>MMRLRGSGMLRDLLLRSPAGVSATLRRAQPLVTLCRRPRGGGRPAAGPAAAARLHPWWGGGGWPAEPLARGLSSSPSEILQELGKGSTHPQPGVSPPAAPAAPGPKDGPGETDAFGNSEGKELVASGENKIKQGLLPSLEDLLFYTIAEGQEKIPVHKFITALKSTGLRTSDPRLKECMDMLRLTLQTTSDGVMLDKDLFKKCVQSNIVLLTQAFRRKFVIPDFMSFTSHIDELYESAKKQSGGKVADYIPQLAKFSPDLWGVSVCTVDGQRHSTGDTKVPFCLQSCVKPLKYAIAVNDLGTEYVHRYVGKEPSGLRFNKLFLNEDDKPHNPMVNAGAIVVTSLIKQGVNNAEKFDYVMQFLNKMAGNEYVGFSNATFQSERESGDRNFAIGYYLKEKKCFPEGTDMVGILDFYFQLCSIEVTCESASVMAATLANGGFCPITGERVLSPEAVRNTLSLMHSCGMYDFSGQFAFHVGLPAKSGVAGGILLVVPNVMGMMCWSPPLDKMGNSVKGIHFCH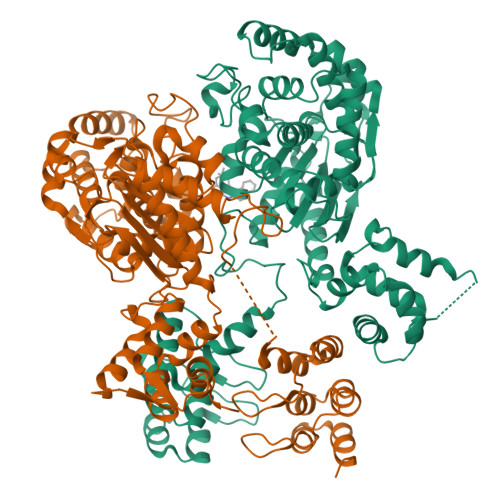DLVSLCNFHNYDNLRHFAKKLDPRREGGDQRVKSVINLLFAAYTGDVSALRRFALSAMDMEQRDYDSRTALHVAAAEGHVEVVKFLLEACKVNPFPKDRWNNTPMDEALHFGHHDVFKILQEYQVQYTPQGDSDNGKENQTVHKNLDGLL[2x]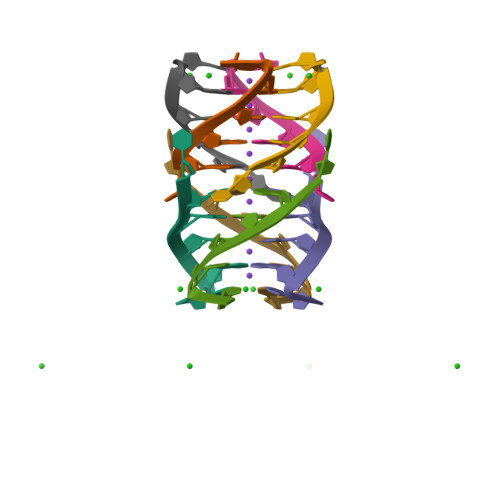>[2x]UGGGGU> MRYIRLCIISLLATLPLA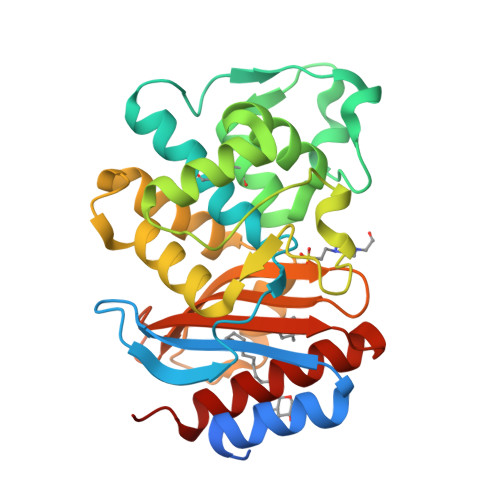VHASPQPLEQIKLSESQLSGRVGMIEMDLASGRTLTAWRADERFPMMSTFKVVLCGAVLARVDAGDEQLERKIHYRQQDLVDYSPVSEKHLADGMTVGELCAAAITMSDNSAANLLLATVGGPAGLTAFLRQIGDNVTRLDHWETELNEALPGDARDTTTPASMAATLRKLLTSQRLSARSQRQLLQWMVDDRVAGPLIRSVLPAGWFIADKTGAGERGARGIVALLGPNNKAERIVVIYLRDTPASMAERNQQIAGIGAALIEHWQR> AATSRDALPNTEASGPTHSKEIPALTAVETGATNPLVPSDTVQTRHVVQHRSRSESSIESFFARGACVTIMTVDNPASTTNKDKLFAVWKITYKDTVQLRRKLEFFTYSRFDMELTFVVTANFTETNNGHALNQVYQIMYVPPGAPVPEKWDDYTWQTSSNPSIFYTYGTAPARISVPYVGISNAYSHFYDGFSKVPLKDQS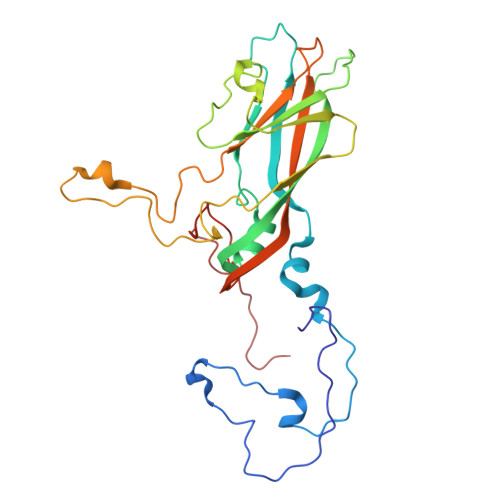AALGDSLYGAASLNDFGILAVRVVNDHNPTKVTSKIRVYLKPKHIRVWCPRPPRAVAYYGPGVDYKDGTLTPLSTKDLTTY>EAALGDAKDALYAALEGMNRGIFGMTSEKRSEIHALVELLESKNPTPEPTDKLQDKVDGCWRLVYSTISILGKKRTKLGLRDFISLGDFFQMIDVKEEKAVNVIKFSARALKILSGQLTIEASYKITTKTKVDITLDSSTITPDQLMNIFQKNYDMLLAIF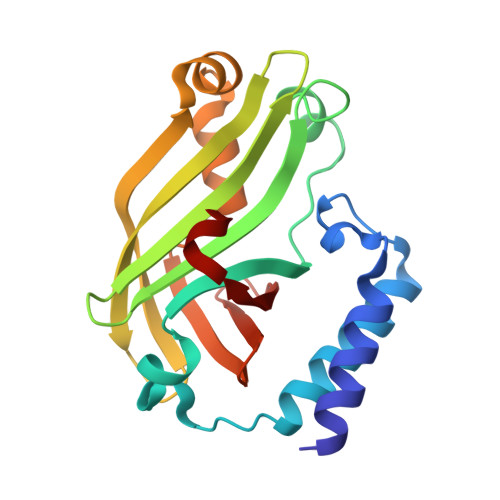NPEGWLEITYVDESLRIGRDDKANIFVLERADPSEV[3x]Mitochondrial ATP synthase uses the energy of the electrochemical proton gradient across the inner mitochondrial membrane to produce ATP from ADP and phosphate by rotary catalysis. ATP synthases consist of the catalytic F1 head and the Fo subcomplex in the membrane. Rotation is driven by protons flowing down the membrane gradient through the Fo subcomplex. A conserved glutamate (cGlu111 in Polytomella) serves as the c-subunit proton-binding site.

We determined the structure of a 1.6 MDa mitochondrial F1Fo ATP synthase dimer by single-particle electron cryo-microscopy. At 3.7 Å resolution, all Fo subunits, helices, loops, most sidechains and some lipids are well resolved. The best-defined region of the assembly includes subunit a, the c-ring interface and ASA 6, which was built de novo. Two prominent aqueous channels defined by subunit a and the 10-subunit c-ring rotor conduct protons to protonate and deprotonate a c-subunit glutamate in the middle of the membrane. The lumenal channel extends to a cluster of buried, closely spaced glutamates and histidines (aGlu172, aHis248, aHis252, aGlu288) that appears to serve as a local reservoir for protons to be fed to the c-ring glutamates. At aGlu288 about 20 Å below the lumenal membrane surface, the channel narrows to 4 by 5 Å and changes direction by 90° towards the c-ring. The matrix channel is defined by the N-terminal half of H5 (residues 221–239), the C-terminal half of H6 (301–312) and residues cTyr102 to cGlu111 of the outer helices of c-subunits A and J. Its deepest point is a 4 Å by 7 Å cavity next to cJGlu111, ~25 Å below the c-ring surface. The positively charged, strictly conserved aArg239 in H5 separates the lumenal and matrix channels, preventing proton leakage. The shortest distance between the lumenal and matrix channels on either side of aArg239 is ~6 Å. Our structure, in particular the small distance between channels, supports the notion that the force generated by the electrostatic field acting on the deprotonated cGlu111 gives rise to directional c-ring rotation.

>MSVQRLSLGAARCLSAGVARVQASQALVAQKAVAVAPTRAQAAPAEVAQVRSMSVLAASKMVGAGCATIALAGVGAGLGVMFGSLINGAARNPNIAKQLVGYALLGFALTESIALFSLLVVFLILFA[10x];> MSVLSSVSMGSRIGSSLLGRSSAYLAQCGFSTRSNLNGSIDTSSSVFQALSSDNENKPAASPLNVKLPGMSCSSILLPKTSRIAVPFGNQTMAMSSVRDVKTGSLPTNFLTGVYRFWRSQNPAEKPHDPVNDRLLPAVVDASDKRASIGTWATTFFCTIISCNLLGLMPFNEAPTSGLGFATGLGVSVWATATILGLSKTGFKFPGHFIPGGTPWPMAFIFVPLETISYTFRAVSLGVRLWVNMLAGHTLLHILTGMALALPFSLGFFSMVPATFGVCCLLSALVGLEYLVAVLQSGVFSILSTVYVGEFNHDKFIGPAAKIVKKIH;> MMLRTLTRSSAVAGQAVRLFKTSAAAAEGNSVAGIIKSVNETSGANLLSSLKTIKAQAAPIYPAAASSTGYSTQAKIALFGALSWILYRADGQSKAHEWIVDLNLNVLQAAWLISFSSLIPFRAVYFAFRGMAPATASTLNGLKTFSSISL>AMAIPAFHPGELNVYSAPGDVADVSRALRLTGRRVMLVPTMGALHEGHLALVRAAKRV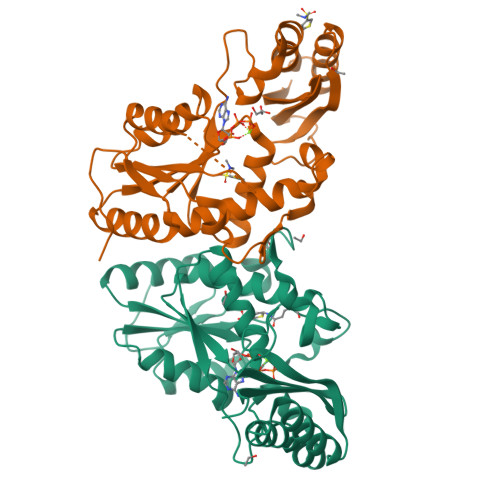PGSVVVVSIFVNPMQFGAGGDLDAYPRTPDDDLAQLRAEGVEIAFTPTTAAMYPDGLRTTVQPGPLAAELEGGPRPTHFAGVLTVVLKLLQIVRPDRVFFGEKDYQQLVLIRQLVADFNLDVAVVGVPTVREADGLAMSSRNRYLDPAQRAAAVALSAALTAAAHAATAGAQAALDAARAVLDAAPGVAVDYLELRDIGLGPMPLNGSGRLLVAARLGTTRLLDNIAIEIGTFAGTDRPDGYR[2x]>[2x]VPRGSHMKKLLVANRGEIAVRVFRACNELGLSTVAVYAREDEYSVHRFKADESYLIGQGKKPIDAYLDIDDIIRVALESGADAIHPGYGLLSENLEFATKVRAAGLVFVGPELHHLDIFGDKIKAKAAADEAKVPGIPGTNGAVDIDGALEFAKTYGYPVMIKAALGGGGRGMRVARNDAEMHDGYARAKSEAIGAFGSGEIYVEKYIENPKHIEVQILGDRHGNIIHLHERDCSVQRRNQKVIEIAPAVGLSPDFRNEICEAAVKLCKNVGYVNAGTVEFLVKDDKFYFIEVNPRVQVEHTITELITGVDIVQAQILIAQGKDLHREIGLPAQSEIPLLGSAIQCRITTEDPQNGFLPDTGKIDTYRSPGGFGIRLDVGNAYAGYEVTPYFDSLLVKVCTFANEFSDSVRKMDRVLHEFRIRGVKTNIPFL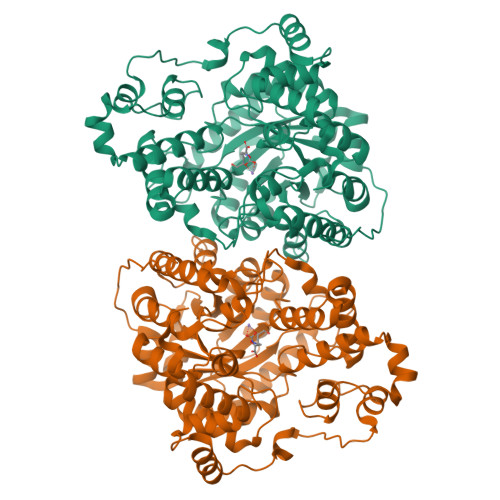INVIANENFTSGQATTTFIDNTPSLFNFPRLRDRGTKTLHYLSMITVNGFPGIENTEKRHFEEPRQPLLNLEKKKTAKNILDEQGADAVVDYVKNTKEVLLTDTTLRDAHQSLLATRLRLQDMKGIAQAIDQGLPELFSAEMWGGATFDVAYRFLNESPWYRLRKLRKLMPNTMFQMLFRGSNAVGYQNYPDNVIEEFIRVAAHEGIDVFRIFDSLNWLPQMEKSIQAVRDNGKIAEATICYTGDILDPSRPKYNIQYYKDLAKELEATGAHILAVKDMAGLLKPQAAYRLISELKDTVDLPIHLHTHDTSGNGIITYSGATQAGVDIIDVATASLAGGTSQPSMQSIYYALEHGPRHASINVKNAEQIDHYWEDVRKYYAPFEAGITSPQTEVYMHEMPGGQYTNLKSQAAAVGLGHRFDEIKQMYRKVNMMFGDIIKVTPSSKVVGDMALFMIQNDLTEEDVYARGNELNFPESVVSFFRGDLGQPVGGFPEKLQKIIVKDKAVITDRPGLHAEKVDFETVKADLEQKIGYEPGDHEVISYIMYPQVFLDYQKMQREFGAVTLLDTPTFLHGMRLNEKIEVQIEKGKTLSIRLDEIGEPDLAGNRVLFFNLNGQRREVVINDQSVQAQVVAKRKAETGNPNQIGATMPGSVLEILVKAGDKVQKGQALMVTEAMKMETTIEAPFDGEIVDLHVVKGEAIQTQDLLIEIN2-((S)-4-(4-chlorophenyl)-2,3,9-trimethyl-6H-thieno[3,2-f][1,2,4]triazolo[4,3-a][1,4]diazepin-6-yl)-N-((1-(4-(2-((2-(2,6-dioxopiperidin-3-yl)-1,3-dioxoisoindolin-4-yl)amino)acetamido)butyl)-1H-1,2,3-triazol-4-yl)methyl)acetamide 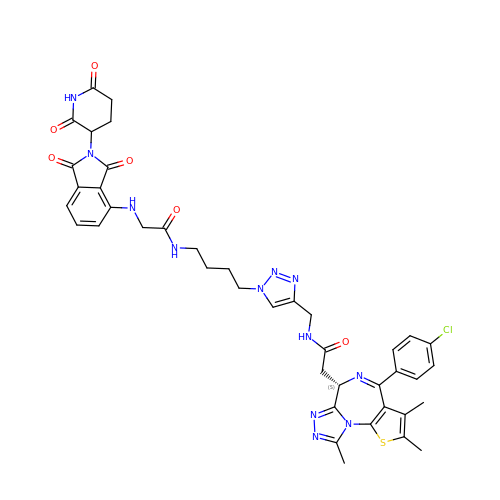| C41 H41 Cl N12 O6 S | RXKCXGDDGPGXLS-UFXYQILXSA-N> DPIANAVENAVSALADTTISRVTAASTAASTHSLGTGRVPALQAAETGASSNASDENLIETRCVMNRNGVNEASVEHFYSRAGLVGVVEVKDSGTSLDGYTVWPIDVMGFVQQRRKLELSTYMRFDAEFTFVSNLNDSTTPGMLLQYMYVPPGAPKPDSRKSYQWQTATNPSVFAKLSDPPPQVSVPFMSPATAYQWFYDGYPTFGEHKQATNLQYGQCPNNMMGHFAIRTVSESTTGKNVHVRVYMRIKHVRAWVPRPLRSQAYMVKNYPTYSQTITNTATDRASITTTDYEGGVPANPQRTS;> MGAQVSTEKSGSHETKNVATEGSTINFTNINYYKDSYAASASRQDFAQDPAKFTRPVLDTIREVAAPLQSPSVEACGYSDRVAQLTVGNSTITTQEAANIVLSYGEWPEYCPSTDATAVDKPTRPDVSVNRFYTLSTKSWKTESTGWYWKFPDVLNDTGVFGQNAQFHYLYRSGFCMHVQCNASKFHQGALLVAAIPEFVVAASSPATKPNGQGLYPDFAHTNPGKNGQEFRDPYVLDAGIPLSQALVFPHQWINLRTNNCATIIMPYVNALPFDSALNHSNFGLVVIPISPLKYCNGATTEVPITLTIAPLNSEFSGLRQAIKQ;> GFPTELKPGTNQFLTTDDGTSPPILPGFEPTPLIHIPGEFTSLLDLCQIETILEVNNTTSTTGVSRLLIPVRAQNNVDQLCASFQVDPGRNGPWQSTMVGQICRYYTQWSGSLKVTFMFTGSFMATGKMLIAYTPPGSAQPATREAAMLGTHIVWDFGLQSSVTLVIPWISNTHFRAVKTGGVYDYYATGIVTIWYQTNFVVPPDTPTEANIIALGAAQKNFTLKLCKDTDEIQQTAEYQ

CVA6 and EV-A71 are both viruses of the Enterovirus genus. P1 harbors the structural proteins that form the capsids, while P2 and P3 encompass the non-structural proteins responsible for the processing and replication of the viral RNA. An example of such a platform is the baculovirus expression vector system (BEVS), requiring only the expression the P1 polyprotein and 3CD protein to produce enterovirus VLPs. Second, native virions have the viral capsid protein VP0 cleaved into VP2 and VP4, whereas VLPs (generally) have VP0 intact.

Single-particle analysis with 44,582 particles yielded an icosahedral CVA6 VLP capsid structure at 3.15 Å overall resolution. The structure of the CVA6 VLP revealed typical surface features associated with enteroviruses, such as the prominent star-shaped plateau (mesa) at the 5-fold-symmetry axes, a narrow canyon-like depression surrounding the mesa, and an open channel situated at the 2-fold axes. Furthermore, the cryo-EM reconstruction revealed that the independent precursors of the particles (protomers) consisting of the three viral proteins (VP0,VP1, and VP3) were highly similar to the previously reported structure. The structure of our CVA6 VLP matched well with those of the CVA6 procapsid (RMSD between 189 pruned atom pairs: 0.729 Å; across all 207 pairs: 1.181 Å) and the previously reported CVA6 VLP (RMSD between 196 pruned atom pairs: 0.917 Å; across all 221 pairs: 1.354 Å). Despite these minor differences between the previously published CVA6 VLP structure and ours, both structures indicated an absence of the pocket factor. The second indication hereof, also deduced from the cryo-EM structure, was the absence of the characteristic VP0 cleavage into VP2 and VP4. With a sequence coverage of >80%, our MS data unequivocally revealed the presence of this concatenated VP0 protein and indicated extremely low concentrations of VP4 and VP2. Our 3D reconstruction and associated radial intensity averages reveal weak, but unstructured, density signal in the particle interior. While previous enterovirus VLP reconstructions did not detect the presence of RNA (center is masked out in the CVA6 structure), we consider the presence of RNA to be the most plausible explanation for this observed increased density, whereby this RNA could change conformation or orientation within the VLP particle. The observed differences in critical force and critical indentation indicate that CVA6 VLPs can withstand less force and deformation prior to structural failure than their virion counterparts.>[6x]MIGVNRMTEASTYIGTVQDVNGANIRVVLDINTISSLKFVDGQGYRIGQIGSFVRIPIGYINLFGIVSQVGAGAVPDKLLEVEPYGHRWISVQLVGEEGIKKEFERGVSQYPTIGDKVHIVTEPDLKKIYGTQNKKYISLGNIASVDSIPALVNIDTLVTRHSAVLGSTGSGKSTTVTSILQRISDMSQFPSARIIVFDIHGEYAAAFKGKAKVYKVTPSNNELKLSIPYWALTCDEFLSVAFGGLEGSGRNALIDKIYELKLQTLKRQEYEGINEDSLTVDTPIPFSIHKLWFDLYRAEISTHYVQGSHSEENEALLLGEDGNPVQKGDSLKVVPPIYMPHTQAQGATKIYLSNRGKNIRKPLEGLASLLKDPRYEFL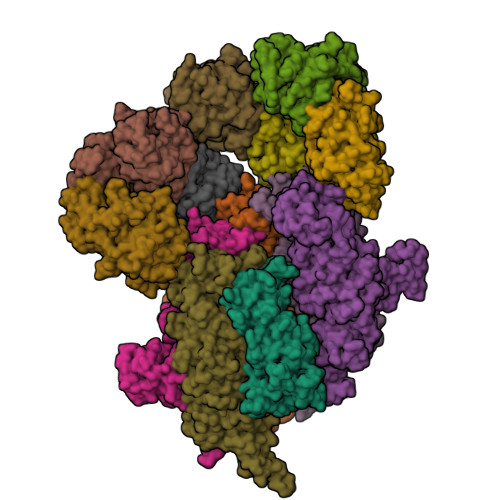FNADDWSVNLDGKTNKDLDALLETWVGSEESISIFDLSGMPSSILDTLIGILIRILYDSLFWSRNQPEGGRERPLLVVLEEAHTYLGKDSRGIAIDGVRKIVKEGRKYGIGMMLVSQRPSEIDSTILSQCGTLFALRMNNSSDRNHVLGAVSDSFEGLMGMLPTLRTGEAIIIGESVRLPMRTIISPPPFGRRPDSLDPDVTAKWSNNRVQGDYKEVLTLWRQKKVRSQRIVENIKRLPVVNEGEMTDMVREMVTSSNILSIGYEADSMTLEIEFNHGLVYQYYDVPETLHTELLAAESHGKFFNSQIKNNYRFSRI;>MDHSITASYYDTTQQLSLLKHVLSEDKRPIAFIIAAGCPVSIRHNDAPLIPDVAGLTRKISDSFGGNPDSLLMKIIQNLKTTIPNPTIEDILSYIRLLQQIPMSGKIHDVENSVINALEESICELIEEEVNVDLPGNATPYHKIAAWINSINREHQVEIFTTNYDLLMEQALEELNVPYFDGFVGSKRAFFDIRTIEENKLPSRWSKLWKLHGSINWQLDKQTQTIWRGTPSKGCSLIHPSHLKYDQSRKMPYLVMMDQLKLFLNQPSAILITCGYSYKDQHINEVLSQGLQTNPNALIYGLQYDVLENYQEAKDMALKRSNLILLAKDRAIIGKKEGEWKPDPQSSQDNDPLLFFKLGDFQHLASFLEEISQYDWSKQND[7x]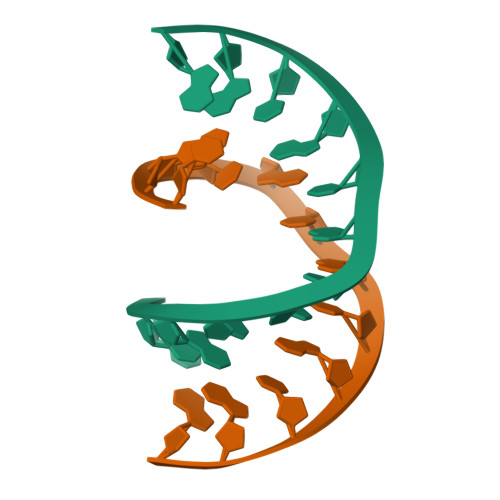>[2x]CTACGCGCGTAG>[4x]APKNELVQKFQVYYLGNVPVAKPVGVDVINGALESVLSSSSREQWTPSHVSVAPATLTILHQQTEAVLGECRVRFLSFLAVGRDVHTFA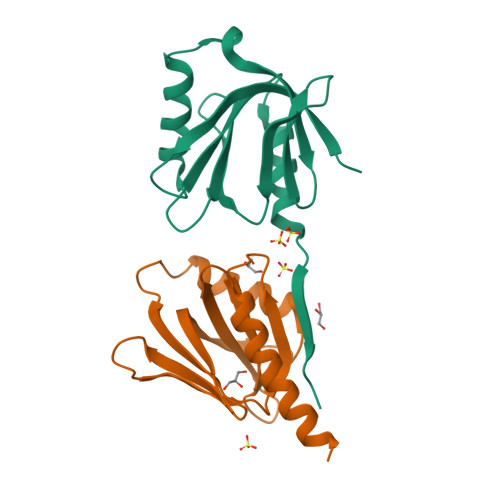FIMAAGPASFCCHMFWCEPNAASLSEAVQAACMLRYQKCLDARSQHHHHHH Immature retroviruses are built by the Gag polyprotein; Gag is then cut into domains, and the resulting CA capsid proteins form the mature capsid, which can mediate infection of a new cell. Murine leukemia virus (MLV), the prototypic member of the γ-retroviruses, is commonly used in comparative studies and as a basis for retroviral vector design. The CA domain and immediate downstream residues mediate protein interactions in the immature shell, and, following proteolytic cleavage, CA forms the mature viral capsid. In this study, we have determined the structure of the truncated MLV CA-CTD by X-ray crystallography and have resolved the architecture and CA lattice structures of immature and mature MLV particles by cryo-ET and subtomogram averaging.

Intermediate- or high-resolution structures have been determined for the immature capsids within a β-retrovirus [Mason–Pfizer monkey virus (M-PMV) (4)] and lentivirus [HIV-1 (4, 5)] as well as for virus-like particles mimicking an immature α-retrovirus [Rous sarcoma virus (RSV) (6)]. Surprisingly, the quaternary structural arrangements of CA domains within the immature lattice again differ significantly among genera: although the arrangement of the CA-CTD appears mostly conserved among RSV, M-PMV, and HIV-1, the CA-NTD arrangements are quite different. The general architecture of the immature MLV lattice is similar to the previously determined HIV-1 and M-PMV Gag shells: it consists of a hexameric arrangement of Gag in which curvature is accommodated by the presence of multiple small defects and one larger defect rather than by Gag pentamers.

>GFDFAVIKELKTAASQYGATAPYTLAIVESVADNWLTPTDWNTLVRAVLSGGDHLLWKSEFFENCRDTAKRNQQAGNGWDFDMLTGSGNYSSTDAQMQYDPGLFAQIQAAATKAWRKLPVKGDPGASLTGVKQGPDEPFADFVHRLITTAGRIFGSAEAGVDYVKQLAYENANPACQAAIRPYRKKTDLTGYIRLCSDIG[3x]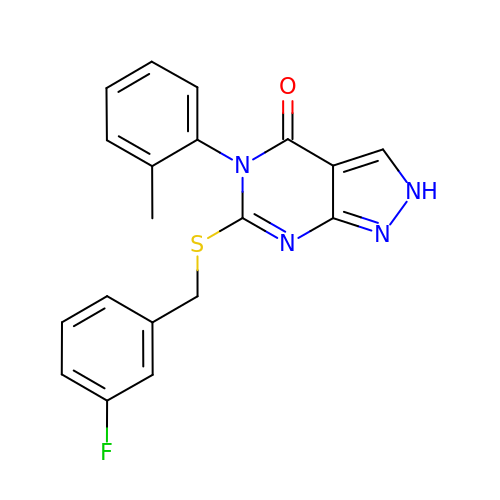6-{[(3-fluorophenyl)methyl]sulfanyl}-5-(2-methylphenyl)-2,5-dihydro-4H-pyrazolo[3,4-d]pyrimidin-4-one | C19 H15 F N4 O S | SSEVBNPAVKLWFQ-UHFFFAOYSA-N> GMNNIIVGMGEALWDVLPEGKKIGGAPANFAYHVSQFGFDSRVVSAVGNDELGDEIMEVFKEKQLKNQIERVDYPTGTVQVTLDDEGVPCYEIKEGVAWDNIPFTDELKRLALNTRAVCFGSLAQRNEVSRATINRFLDTMPDIDGQLKIFDINLRQDFYTKEV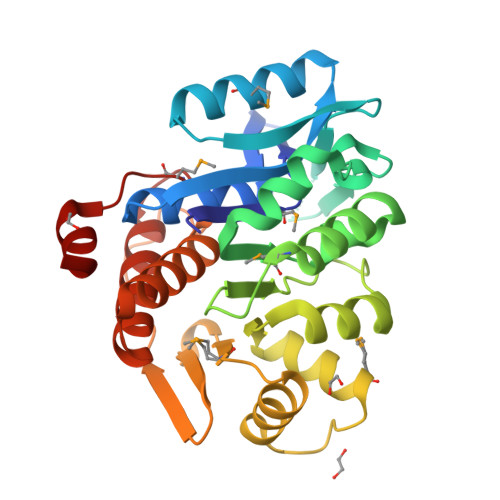LRESFKRCNILKINDEELVTISRMFGYPGIDLQDKCWILLAKYNLKMLILTCGINGSYVFTPGVVSFQETPKVPVADTVGAGDSFTAAFCASILNGKSVPEAHKLAVEVSAYVCTQSGAMPELPVILKDRLL> SNAMKILLRNALITNEGKT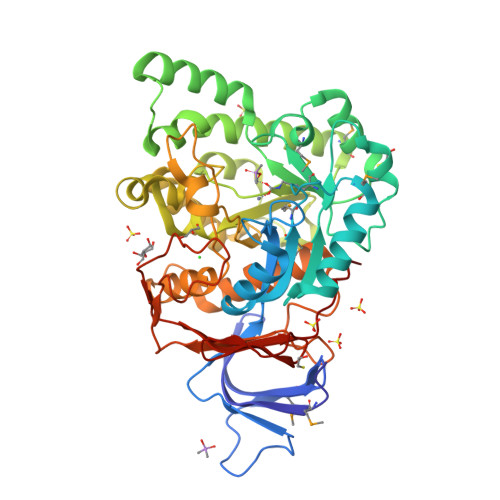FPGSVMIDGAFISRIIEGELPADDNLSADEVIECSGLRLFPGCIDDQVHFREPGLTHKATIASESRAAVAGGVTSFMDMPNTNPPTTMWERLLEKRQIGADTAWANYGFFFGGTNDNIDEIKRVDKHLVPGLKLFLGSSTGNMLVDNKETLEKIFGECDLLIATHCEKEEIIRANKEHYKAKYGNDLDIHFHPLIRSEEACYRSSAEAVELAERMNARLHILHLSTEKELSLFRNDIPTAQKRITSEVCVHHLWFSDTDYGRLGNRIKWNPAIKKESDREALRAAVRNGRIDIIATDHAPHLLREKEGSCLQAASGGPLVQHSLLALLELCNQGIFSIEEIVSKTAHIPATLFAIEKRGYIRPGYYADLVLVDPSSPHTVSADNILSLCGWSPFEGFTFSHSVAYTFVNGCLAYAKGRLAESRPTVHPLFFNR>[2x]MAPHGDGLSDIEEPEVDAQSEILRPISSVVFVIAMQAEALPLVNKFGLSETTDSPLGKGLPWVLYHGVHKDLRINVVCPGRDAALGIDSVGTVPASLITFASIQALKPDIIINAGTCGGFKVKGANIGDVFLVSDVVFH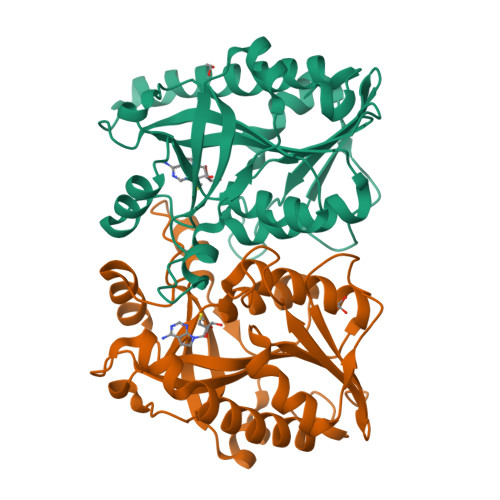DRRIPIPMFDLYGVGLRQAFSTPNLLKELNLKIGRLSTGDSLDMSTQDETLIIANDATLKDMEGAAVAYVADLLKIPVVFLKAVTDLVDGDKPTAEEFLQNLTVVTAALEGTATKVINFINGRNLSDL> ARDSLREELVITPLPSGDVAATFQFRTRWDSELQREGVSHYRLFPKALGQLISKYSLRELHLSFTQGFWRTRYWGPPFLQAPSGAELWVWFQDTVTDVDKSWKELSNVLSGIFCASLNFIDSTNTVTPTASFKPLGLANDTDHYFLRYAVLPREVVCTENL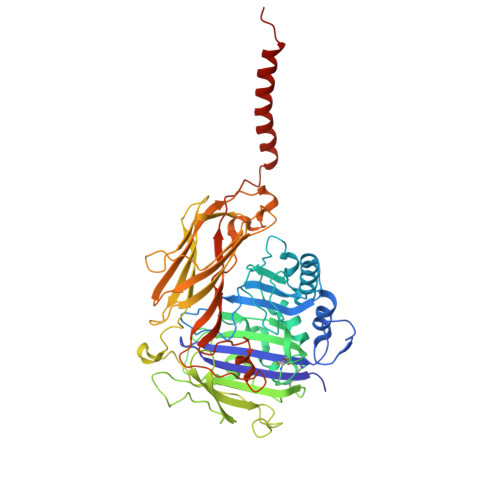TPWKKLLPCSSKAGLSVLLKADRLFHTSYHSQAVHIRPVCRNARCTSISWELRQTLSVVFDAFITGQGKKDWSLFRMFSRTLTEPCPLASESRVYVDITTYNQDNETLEVHPPPTTTYQDVILGTRKTYAIYDLLDTAMINNSRNLNIQLKWKRPPENEAPPVPFLHAQRYVSGYGLQKGELSTLLYNTHPYRAFPVLLLDTVPWYLRLYVHTLTITSKGKENKPSYIHYQPAQDRLQPHLLEMLIQLPANSVTKVSIQFERALLKWTEYTPDPNHGFYVSPSVLSALVPSMVAAKPVDWEESPLFNSLFPVSDGSNYFVRLYTEPLLVNLPTPDFSMPYNVICLTCTVVAVCYGSFYNLLTRTFH> LQDQYKEGIKVVDIDDPDMMVDSFTMPNISHSNIDYQTLLANSDHAKFTIEPGVLPVGIDTHTATDIYQTLIALNLDTTVNDCLDKLLNDECTESTRENALYDYYALQLLPLQKAVRGHVLQFEWHQNSLLTNTHPNFLSKIRNINVQDALLTNQLYKNHELLKLERKKTEAVARLKSMNKSAINQYNRRQDKKNKRLKFGHRLIATHTNLERDEQKRAEKKAKERLQALKANDEEAYIKLLDQTKDTRITHLLRQTNAFLDSLTRAVKDQQKYTKEMIDSHIKEASEEVDDLSMVPKMKDEEYDDDDDNSNVDYYNVAHRIKEDIKKQPSILVGGTLKDYQIKGLQWMVSLFNNHLNGILADEMGLGKTIQTISLLTYLYEMKNIRGPYLVIVPLSTLSNWSSEFAKWAPTLRTISFKGSPNERKAKQAKIRAGEFDVVLTTFEYIIKERALLSKVKWVHMIIDEGHRMKNAQSKLSLTLNTHYHADYRLILTGTPLQNNLPELWALLNFVLPKIFNSVKSFDEWFNTPFANTGGQDKIELSEEETLLVIRRLHKVLRPFLLRRLKKDVEKELPDKVEKVVKCKMSALQQIMYQQMLKYRRLFIGDQNNKKMVGLRGFNNQIMQLKKICNHPFVFEEVEDQINPTRETNDDIWRVAGKFELLDRILPKLKATGHRVLIFFQMTQIMDIMEDFLRYINIKYLRLDGHTKSDERSELLRLFNAPDSEYLCFILSTRAGGLGLNLQTADTVIIFDTDWNPHQDLQAQDRAHRIGQKNEVRILRLITTNSVEEVILERAYKKLDIDGKVIQAGKFDNKSTSEEQEALLRSLLDAEEERRKKRESGVEEEEELKDSEINEILARNDEEMAVLTRMDEDRSKKEEELGVKSRLLEKSELPDIYSRDIGAELKREESESAAVYNGRGARERKTATYNDNMSEEQWLRQFEVSDDEKNDKQARKQRTKKEDKSEAIDGGGSGGHHHHHH;> SNQLISNYAASNSMDRSSSASNEFVPNTSDNNNNSNNHNMRNNSNNKTSNNNNVTAVPAATPANTNNSTSNANTVFSERAAMFAALQQKQQQRFQALQQQQQQQQNQQQQNQQPQQQQQQQQNPKFLQSQRQQQQRSILQSLNPALQEKISTELNNKQYELFMKSLIENCKKRNMPLQSIPEIGNRKINLFYLYMLVQKFGGADQVTRTQQWSMVAQRLQISDYQQLESIYFRILLPYERHMISQEGIKETQAKRIFLQQFLQELLKKVQQQQQAAALANANNNINSASSAPTPAAPGASVPATAAPGTEAGIVPVSANTPKSLNSNININVNNNNIGQQQVKKPRKQRVKKKTKKELELERKEREDFQKRQQKLLEDQQRQQKLLLETKLRQQYEIELKKLPKVYKRSIVRNYKPLINRLKHYNGYDINYISKIGEKIDSNKPIFLFAPELGAINLHALSMSLQSKNLGEINTALNTLLVTSADSNLKISLVKYPELLDSLAILGMNLLSNLSQNVVPYHRNTSDYYYEDAGSNQYYVTQHDKMVDKIFEKVNNNATLTPNDSNDEKVTILVDSLTGNQLPTPTPTEMEPDLDTECFISMQSTSPAVKQWDLLPEPIRFLPNQFPLKIHRTPYLTSLKKIKDEIDDPFTKINTRGAEDPKVLINDQLSTISMILRNISFSDNNSRIMSRNFYLKRFISDLLWLVLIHPENFTCNRKILNFKKDLVIVLSNISHLLEIASSIDCLLILILVISFGQPKLNPMASSSSFGSESLTFNEFQLQWGKYQTFGVDILAKLFSLEKPNLNYFKSILLNKNTGNNLYDRNSNNNHKDKKLLRRLLNLYNDNNKNNNNRHNLLNDVVSFLFSAIPLQQVLSQSADPSLLIDQFSPVISQSLTSILVIVQKILPLSNEVFEISENNSDSNSNNNGNKDSSFNFNKNLPFVWLSSEENIGSGLLKLSEIILNINNSTSKNTLLQQQNYSKVLLPSINISCVQLIKCLVEKSICFENCLNNDPEILKKIASIPNLFPTDLEIFQLFTNPSVDIQIINQYQLLYNLKNDILTNLEGGSGGWSHPQFEKWSHPQFEKWSHPQFEK;> MNNQPQGTNSVPNSIGNIFSNIGTPSFNMAQIPQQLYQSLTPQQLQMIQQRHQQLLRSRLQQQQQQQQQTSPPPQTHQSPPPPPQQSQPIANQSATSTPPPPPAPHNLHPQIGQVPLAPAPINLPPQIAQLPLATQQQVLNKLRQQAIAKNNPQVVNAITVAQQQVQRQIEQQKGQQTAQTQLEQQRQLLVQQQQQQQLRNQIQRQQQQQFRHHVQIQQQQQKQQQQQQQHQQQQQQQQQQQQQQQQQQQQQQQQQQQQQQQQQQQQQGQIPQSQQVPQVRSMSGQPPTNVQPTIGQLPQLPKLNLPKYQTIQYDPPETKLPYPTYWSDKKADTDTLLYEQIIQRDKINKYSLIRETNGYDPFSIYGFSNKEYISRLWHTLKYYQDLKNTRMKSITSTSQKIPSASIWGNGYSGYGNGITNTTTRVIPQVEVGNRKHYLEDKLKVYKQAMNETSEQLVPIRLEFDQDRDRFFLRDTLLWNKNDKLIKIEDFVDDMLRDYRFEDATREQHIDTICQSIQEQIQEFQGNPYIELNQDRLGGDDLRIRIKLDIVVGQNQLIDQFEWDISNSDNCPEEFAESMCQELELPGEFVTAIAHSIREQVHMYHKSLALLGYNFDGSAIEDDDIRSRMLPTITLDDVYRPAAESKIFTPNLLQISAAELERLDKDKDRDTRRKRRQGRSNRRGMLALSGTSASNTSMNGVHNTVAAGNASSLPPGEILLPDIADIPRTFRTPVPSTLMPGGVDVGPSVESYELRNTTTYKSRPDRPKPVSPPCYIIDHIPGHSLLLSIKLPGKVNTKEEFAAAPNDTSSGTNAMLPSPESLKTKLNSNIRAGVTIPSIPNPIANHTVTNSPNPTLQPVIPGGAASKSVPTPSLPIAPPVAPHDSEATLLTNSNNGSSNNNTQNTGGSGGDYKDDDDK;>[2x]MENTLGEGSTVNASVDVDQHGNDNNSDSNANAAVAGVANTDTAGEESQQQDESLKDEATVPNTRDAESEAITVTAKQQPTMQANKLDSQETPSTEESRAQNVFGQDNEDSDNLFGETESSVSNNEANTPSIPTNPVDNENNKPAIKEDSTIQDSNGDVKNMEDVKIQKEEEPENNTVIEGVKEESQPDENTKEMDEVEEDDEDDDQPMISPDNSIFGDTKSESKQLGNTSSVANTPSEIPDAHKAEQEDIIEKTESVDKKVDSGEERNEQEREIMN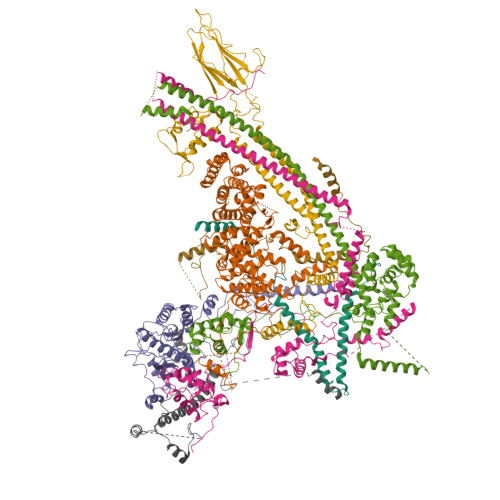DHSKSANPKKTTITRVEPETFEIPQAHEIVIPSYSKWFNLEKIHSIEVQSLPEFFTNRIPSKTPEVYMRYRNFMVNSYRLNPNEYFSVTTARRNVSGDAAALFRLHKFLTKWGLINYQVDSKLLPKNIEPPLTSQYSTRHDAPRGLFPFESYKPSVQLPDMAKLKKMMNTSDSESTLYKYLKESKRKYDEITHPPSTTDDENGDKNDNGGKMNNEVSTSTSMTGDANLLEEGETSRPLKKVKILEQIDENWSKEDLQKLLKGIQEFGADWYKVAKNVGNKSPEQCILRFLQLPIEDKFLYGDGNGKGDNDNGLGPLKYAPHLPFSKSENPVLSTIAFLVGLVNPKTVQSMTQRAIQSAESIKSQKEEISDQKPIEHIKEGSEIAISSLGYRSHIFATNEERQMNFLTNELIRLQMEKLDAKLNHLKKLEKFMELERKTLERQQENLLIQRLNFNQNSSKIVNVLSKCLNLISDSNINNSSVAEKEEIRSQIDHFKSMLSKPETLSIGKNPFNKPNIETGENHNGQSISNENDVKPISIEAPQFYRYWSAGGSGGHHHHHH;> MSKVMKPSNGKGSRKSSKAATPDTKNFFHAKKKDPVNQDKANNASQITPTVPHSHPSDMVIPDHLAELIPELYSFQQLVDSEKRLDHFIHLRNLHMKRMVAQWERSKLSQEFLYPHLNFPNVKFLRIFISNVSENQPWQMDTNNEADLMALENATWTMRIEGRLLDNVQANDPAREKFSSFIESIVVDFKNKENDNVPSTKFNAAPEENATEGPSDKKLNLNLPLQFSLPNGDNSTTTNTDQNNATMGEETAKKDMSSTTPKLESVKWQYDPNNPVDFDGLDIKRVGSENVECTISILRKSSPEEPFMSYSPQLTAIIGLKSGTSHDAIFSIYKYIHLNELLTNDESAFENLMGNRNNHNSNTSTSKMLDAASSQVSIVKLDTQLITLLPSSLKESSPDTMKLTDLLSLINSTHLLPLQPIEIDYTVRVDKASTYGELVLDIEVPDVNALKFNNTQRESQIGAAELNENARELEQIKPKIALQDKEITSVLSNLHESNKRYRFFKKISEDPVKALNECIASTSNALKVLSGDEGYNEDMVRRANFYKENEAMLRENIEVILSNGRM;> MGVIKKKRSHHGKASRQQYYSGVQVGGVGSMGAINNNIPSLTSFAEENNYQYGYSGSSAGMNGRSLTYAQQQLNKQRQDFERVRLRPEQLSNIIHDESDTISFRSNLLKNFISSNDAFNMLSLTTVPCDRIEKSRLFSEKTIRYLMQKQHEMKTQAAELQEKPLTPLKYTKLIAAAEDGSRSTKDMIDAVFEQDSHLRYQPDGVVVHRDDPALVGKLRGDLREAPADYWTHAYRDVLAQYHEAKERIRQKEVTAGEAQDEASLQQQQQQDLQQQQQVVTTVASQSPHATATEKEPVPAVVDDPLENMFGDYSNEPFNTNFDDEFGDLDAVFF;> MLGEDEGNTVLEKGNNPSVKQGEVGAVFIVPKILIREHERVILKQILQILDQDELVQPPLDKFPYKKLELPKYIDELKTRDATNTSYKMIQLDAYGEKKVGSNGELFGGRHYLFNTFTFTAHMGVLLVLLQDVIKVLYQSNATHDEDEFIVQHDQILVMETSEEQTKFLAKNGVIPEESKGSFKYITARSAFVEFGASVIAGGQRIVDDYWESLAKKQNLSSHQRVFKLSTNLISKISLLRPSFQNNRISNANEISANTNNTCTISTSKFESQYPIVTEQPSAEIREAYIENFAKGEHISAIVPGQSISGTLELSAQFRVPRYHSKNSFQQALQMKAMDIPIGRHEELLAQYESQAPDGSASISLPNHIPSVNPSNKPIKRMLSSILDINVSSSKNKKSEENEMIKPMNKGQHKNNTSLNINGWKFESLPLKSAENSGKQQYYRGLPLYEKNTLLERLKQLTPNEIKELEHLHDAVFVNTGLQNVRKVRTKKWKKYWQYKAGIPIGLKRSQLDEFKNKYLKDVLAQTSVTTNFNEITNTDETITTKRVPNPNFLGNCNIKDFKPPYIYSHVNKVPQNVAGDKTAVKLDTEVKNTNANPVVATDPVAAKPDNLANFSNEVAMNNGGSGGHHHHHH>MGNSGFYLYNTENCVFADNIKVGQMTEPLKDQQIILGTKSTPVAAKMTASDGISLTVSNNSSTNASITIGLLKAFNNFPITNKIQCNGLFTPSNIETLLGGTEIGKFTVTPKSSGSMFLVSADIIASRMEGGVVLALVREGDSKPCAISYGYSSGVPNLCSLRTSITNTGLTPTTYSLRVGGLESGVVWVNALSNGNDILGITNTSN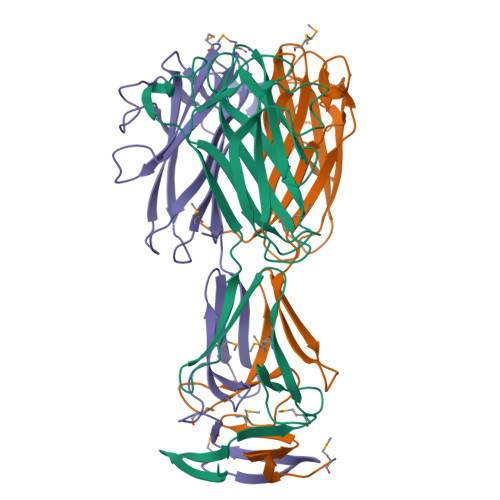VSFLEVIPQTNA[9x]> MAKREPIHDNSIRTEWEAKIAKLTSVDQATKFIQDFRLAYTSPFRKSYDIDVDYQYIERKIEEKLSVLKTEKLPVADLITKATTGEDAAAVEATWIAKIKAAKSKYEA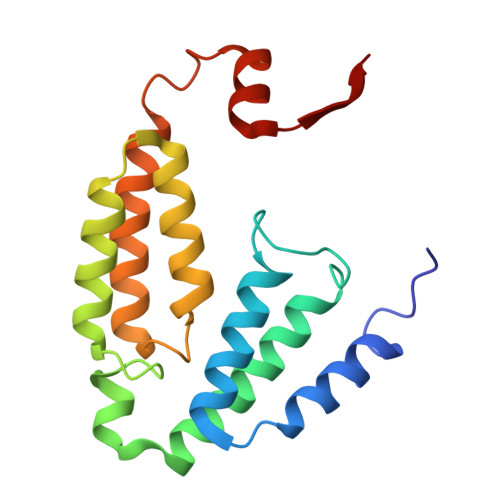ERIHIEFRQLYKPPVLPVNVFLRTDAALGTVLMEIRNTDYYGTPLEGLRKERGVKVLHLQA> SMDSSALPDPGFQKITLSSSSEEYQKVWNLFNRTLPF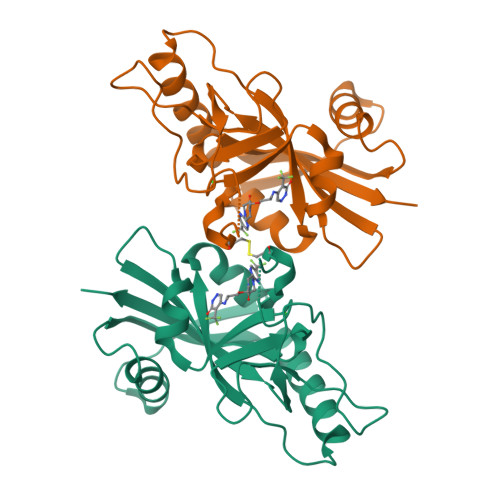YFVQKIERVQNLALWEVYQWQKGQMQKQNGGKAVDERQLFHGTSAIVVDGICQHNFDWRVCGVHGTSYGKGSYFARDAAYSHHFSKSDTQTHTMFLARVLVGEFVRGNASFVRPPAKEGWSNAFYDSCVNSVSDPSIFVIFEKHQVYPEYVIQYTTSSKPS>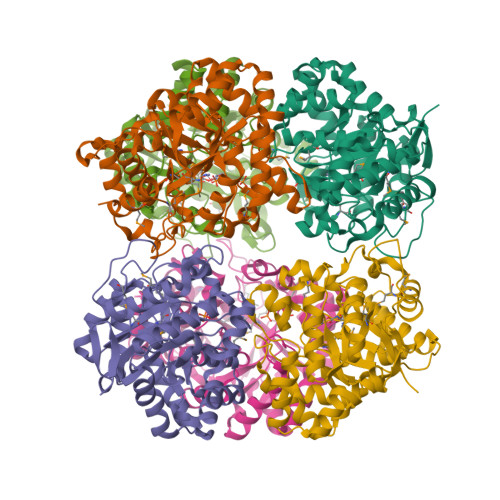[6x]MSLENKFARTVLGDIPVEKLGITDCHDHFIKNGGPEVEEHIDFLMLNVDASIKEFKEFIDRGGSTIVTMDPPNVGRDVLKTLEIANAVKNLGGNVIMSTGFHKAKFYDKYSSWLAVVPTEEIVKMCVAEIEEGMDEYNYNGPVVKRSKAKAGIIKAGTGYGAIDRLELKALEVAARTSILTGCPILVHTQLGTMALEVAKHLIGFGANPDKIQISHLNKNPDKYYYEKVIKETGVTLCFDGPDRVKYYPDSLLAENIKYLVDKGLQKHITLSLDAGRILYQRNYGLTKGKQTFGLAYLFDRFLPLLKQVGVSKEAIFDILVNNPKRVLAFDEKRNFDPLKVSKEVLELKKELNLNEGHHHHHH In this study, we have determined the crystal structures of bcPadR1 and bcPadR2, which are the products of gene loci BC4206 and BCE3449 of B. cereus strains ATCC 14579 and ATCC 10987, respectively. The bcPadR1 and bcPadR2 subunits contain a typical wHTH DNA-binding domain, consisting of helices α1, α2, the DNA recognition helix α3 and strands β1 and β2 (together forming the wing), and a dimerization domain, including the C-terminal helix α4. Unlike LmrR, but like the other PadR-s2 proteins with known structure, the bcPadR1 and bcPadR2 dimers have a completely closed dimer interface. The closed dimer conformation and inaccessibility of the conserved tryptophan residues of the bcPadR proteins are incompatible with a drug-binding mechanism as observed in LmrR.

In addition, we report the crystal structure of a bcPadR1 homolog from B. cereus strain ATCC 10987, the product of gene locus BCE3449, which we named bcPadR2. This latter protein was selected for structural characterization because its gene is positioned in the vicinity of two genes encoding a putative antibiotic ABC efflux pump (gene loci BCE3447 and BCE3446). The proximity of these genes, similar as in the lmrR-lmrCD locus, could indicate that bcPadR2 regulates the expression of the ABC efflux pump, perhaps following a similar ligand binding and induction mechanism as LmrR. The gene encoding bcPadR2 (locus BCE3449 in B. cereus ATCC 10987) lies downstream from two genes, BCE3447 and BCE3446, which encode a putative ABC-efflux pump. Interestingly, the amino acid sequence of the BCE3447-BCE3346 encoded pump is similar to that of the daunorubicin/doxorubicin resistance ABC transporter DrrAB from Streptomyces peucetius (overall sequence identity of 32%). DNA analysis indicates that the BCE3449 and BCE3447-BCE3346 genes do not share a common promoter, and are separated by another gene, BCE3448, which encodes a soluble protein of unknown function. Similarly, bcPadR2 was crystallized in space group P43212, with one protein molecule per asymmetric unit and a solvent content of 42%. In addition, residues 67–71 in the β-wing of bcPadR2 were found to be disordered and therefore left out from the model. Likewise, the bcPadR2 dimer can be fitted to the DNA-bound complexes of RTP and BlaI with RMSD values of 2.9 Å (for 179 common Cα atoms) and 3.4 Å (for 155 common Cα atoms).

> MENLTEMLKGSLEGCVLEIISRRETYGYEITRHLNDLGFTEVVEGTVYTILVRLEKKKLVNIEKKPSDMGPPRKFYSLNEAGRQELELFWKKWDFVSSKINVLKSSNSRWSHPQFEK>[4x]GSHMTETVTETTAPASPEADVQGPDFAAMLAARLCHDFISPASAIVSGLDLLEDPSA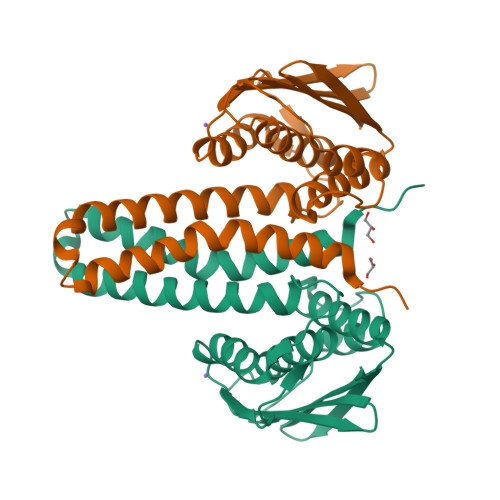QDMRDDAMNLIASSARKLADLLQFTRVAFGASASAENFDSRELEKLAQGVFAHVRPTLDWQIEPQAMNKPSSRAVLNIAQIAASALPAGGVATVKGVAADGRFSIIADAKGPRARLRPEVLAGLKGEPLAEGLGGPWVQAAYLNALVRAAGGQIAVEIGEDRASIAAWVPA>[6x]MAELRERLLRAARWILLLGLLVLVGFVVLAYLERSPLIRAFVLSAGVVLVALFAAALAWLYLAAALLGRSPLLALVALALGLITLAAASAAMAATFAHLLLEAPPEYREAMLYVFGIAVLIVGLLLLGLVWLLEEALEALLEEEKRREEEEKRRELVKRAEEALQKAQEAEKQGDVEKAVKAAQEAVRAAKESGDNDVLRRVAE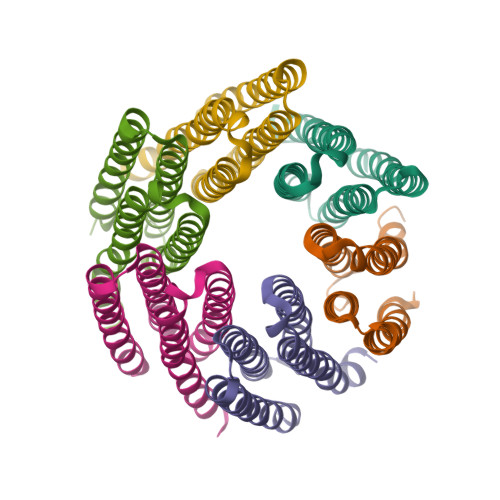QALQIAKEAEKQGNVEVAVKAARVAVEAAKQAGDNDVLRKVAEQALRIAKEAEKQGNVEVAVKAARVAVEAAKQAGDQDVLRKVSEQAERISKEAKKQGNSEVSEEARKVADEAKKQTGGSGGSHHHHHH> MNMFFRLTALAGLLAIAGQTFAVEDITRADQIPVLKEETQHATVSERVTSRFTRSHYRQFDLDQAFSAKIFDRYLNLLDYSHNVLLASDVEQFAKKKTELGDELRSGKLDVFYDLYNLAQKRRFERYQYALSVLEKPMDFTGNDTYNLDRSKAPWPKNEAELNALWDSKVKFDELSLKLTGKTDKEIRETLTRRYKFAIRRLAQTNSEDVFSLAMTAFAREIDPHTNYLSPRNTEQFNTEMSLSLEGIGAVLQMDDDYTVINSMVAGGPAAKSKAISVGDKIVGVGQTGKPMVDVIGWRLDDVVALIKGPKGSKVRLEILPAGKGTKTRTVTLTRERIRLEDRAVKMSVKTVGKEKVGVLDIPGFYVGLTDDVKVQLQKLEKQNVSSVIIDLRSNGGGALTEAVSLSGLFIPAGPIVQVRDNNGKVREDSDTDGQVFYKGPLVVLVDRFSASASEIFAAAMQDYGRALVVGEPTFGAGTVQQYRSLNRIYDQMLRPEWP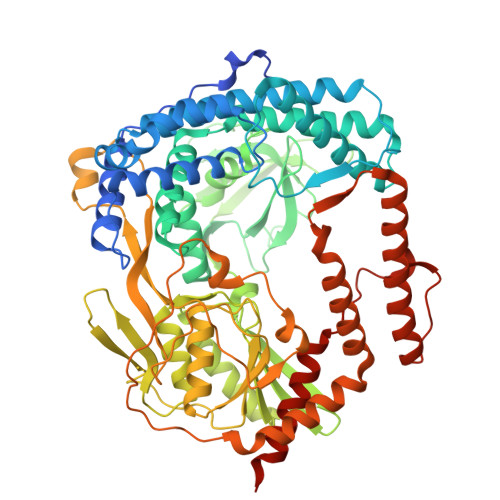ALGSVQYTIQKFYRVNGGSTQRKGVTPDIIMPTGNEETETGEKFEDNALPWDSIDAATYVKSGDLTAFEPELLKEHNARIAKDPEFQNIMKDIARFNAMKDKRNIVSLNYAVREKENNEDDATRLARLNERFKREGKPELKKLDDLPKDYQEPDPYLDETVNIALDLAKLEKARPAEQPAPVK>MKNFRLSEKEVKTLAKRIPTPFLVASLDKVEENYQFMRRHLPRAGVFYAMKANPTPEILSLLAGLGSHFDVASAGEMEILHELGVDGSQMIYANPVKDARGLKAAADYNVRRFTFDDPSEIDKMAKAVPGADVLVRIAVRNNKALVDLNTKFGAPVEEALDLLKAAQDAGLHAMGICFHVGSQSLSTAAYEEALLVARRLFDEAEEMGMHLTDLDIGGGFPVPDAKGLNVDLAAMMEAINKQIDRLFPDTAVWTEPGRYMCGTAVNLVTSVIGTKTRGEQPWYILDEGIYGCFSGIMYDHWTYPLHCFGKGNKKPSTFGGPSCDGIDVLYRDFMAPELKIGDKVLVTEMGSYTSVSATRFNGFYLAPTIIFEDQPEYAARLTEDDDVKKKAAV[2x]

In particular, l-lysine decarboxylase (LDC) is an important enzyme for the biosynthesis of cadaverine, which is a crucial platform chemical with many industrial applications. In this report, we determined the crystal structures of LDC from Selenomonas ruminantium (SrLDC) in different crystallization conditions and observed that high flexibility of the PLP binding site seems to be one of the factors that lead to the low affinity for PLP in SrLDC. The monomeric form of SrLDC consists of two distinct domains, a PLP-binding barrel domain, and a sheet domain. The SrLDC homodimer is formed by a head-to-tail contact between the barrel domain of one monomer and the sheet domain of the other monomer.

To investigate the conformational changes at the active site of SrLDC, we determined its crystal structure in the apo-form with a C2 space group at 2.9 Å resolution. Unlike the two crystal forms described above, the structure contains a dimer in an asymmetric unit. Interestingly, two SrLDC monomers in the asymmetric unit exhibit completely different conformations at the active site, although no cofactor or substrate is bound in either monomer. In one monomer, the PS-loop is in the open-conformation and the R-loop is disordered. In contrast, the other monomer contains both the PS-loop and the R-loop in the closed-conformation observed in the structure of SrLDC complexed with PLP/cadaverine. Moreover, the entire AS-loop is in an ordered-conformation with a clear electron density map in this region. These observations indicate that the open-closed conformation of SrLDC is caused mainly by the different crystal packings rather than by the binding of the PLP cofactor and/or the lysine substrate. In fact, the PS-loop, the R-loop, and the AS-loop all show a much higher b-factor compared with the rest of the protein, indicating that these loop regions are highly flexible. Taken together, the results allow us to conclude that the active site of SrLDC has an extremely high flexibility.> MGNCLDSSAKVDNSNHSPHANSASSGSKVSSKTSRSTGPSGLSTTSYSTDSSFGPLPTLRTEGEILSSPNLKAFTFNELKNATKNFRQDNLLGEGGFGCVFKGWIDQTSLTASRPGSGIVVAVKQLKPEGFQGHKEWLTEVNYLGQLSHPNLVLLVGYCAEGENRLLVYEFMPKGSLENHLFRRGAQPLTWAIRMKVAVGAAKGLTFLHEAKSQVIYRDFKAANILLDADFNAKLSDFGLAKAGPTGDNTHVSTKVIGTHGYAAPEYVATGRLTAKSDVYSFGVVLLELISGRRAMDNSNGGN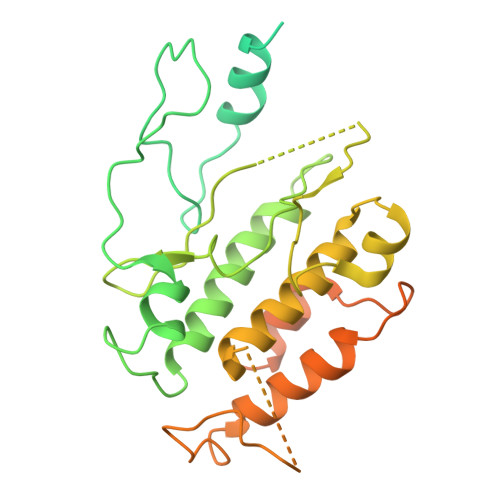EYSLVDWATPYLGDKRKLFRIMDTKLGGQYPQKGAFTAANLALQCLNPDAKLRPKMSEVLVTLEQLESVAKPGTKHTQMESPRFHHSSVMQKSPVRYSHDRPLLHMTPGASPLPSYTQSPRVR> RSDDD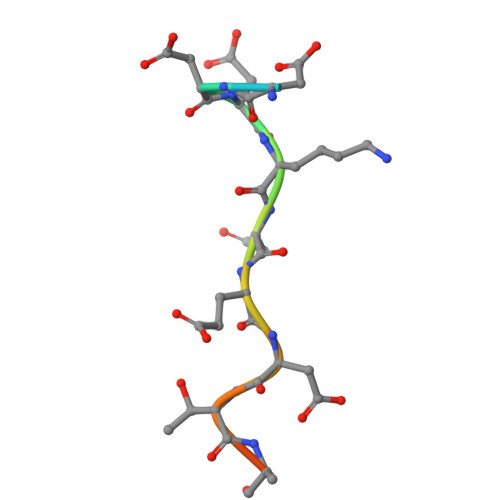KDEDTHSRK> CAGTTGAAAG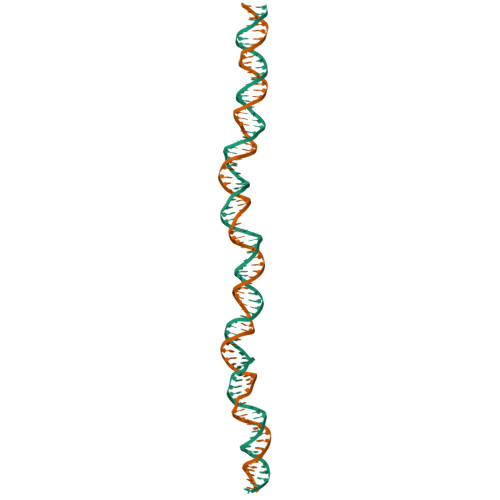TCTTTTTTCTTGCCAGAAAGAATTGGTTTTTCAGCATATAACATCTCACAAAATCACGTTTTCCCTGTTTGATTACCTTTTCT;> AGAAAAGGTAATCAAACAGGGAAAACGTGATTTTGTGAGATGTTATATGCTGAAAAACCAATTCTTTCTGGCAAGAAAAAAGACTTTCAACTG>[2x]GHML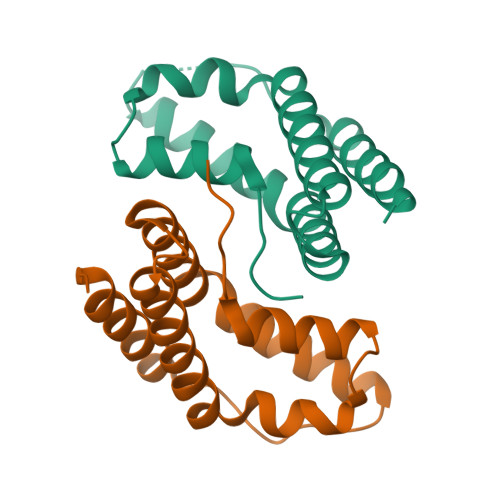YINSFLDRMGEIIRGEKSVEEADKLLDQKNIFEMFRSDCEEILNLYKSGKAEKEEVQRNFYLLKTYVVSQLSIHFERLKEFAESKGFKIEKKLDPEVINEIALYIDRVEKEV(8alpha,9beta,10alpha,13alpha)-13-{[beta-D-glucopyranosyl-(1->2)-[beta-D-glucopyranosyl-(1->3)]-beta-D-glucopyranosyl]oxy}kaur-16-en-18-oic acid | C38 H60 O18 | 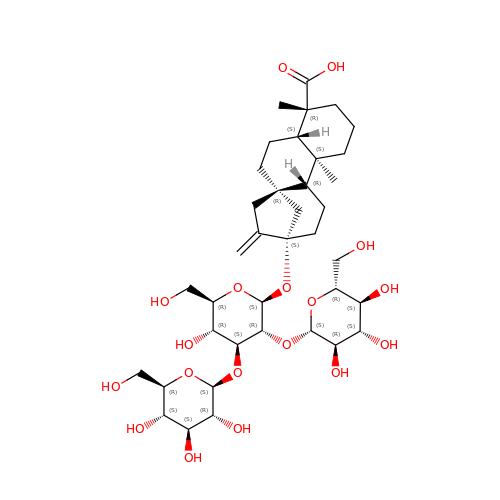DRSKVOAJKLUMCL-MMUIXFKXSA-N>[2x]SAKEYALSGRELT;>[2x]MAFNKDQDYWANIFVTPDFLSVETYSG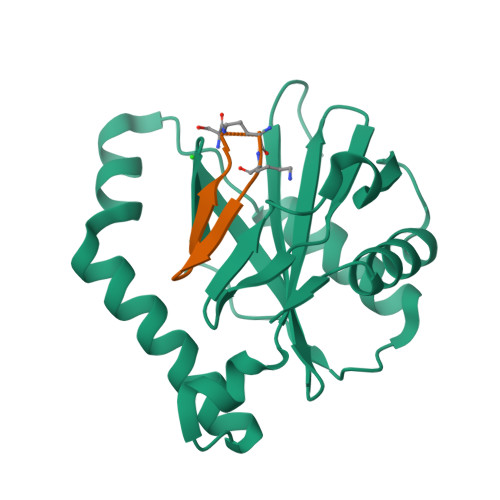LGMTGRDPLFSPRLLQPDVDDKSLGEEILQALSDSRTLDVLEERVAFFDLEKSKEQYAAWIATLMEKYGYRTKRALFKNMKKVGIHLVNDVITIRPSFHEKLEAWSGNRINESDYVVLPADSSPTEIGSGLRLALSRCKGTSLEHHHHHH>LVASGENKIKQGLLPSLEDLLFYTIAEGQEKIPVHKFITALKSTGLRTSDPRLKECMDMLRLTLQTTSDGVMLDKDLFKKCVQSNIVLLTQAFRRKFVIPDFMSFTSHIDELYESAKKQSGGKVADYIPQLAKFSPDLWGVSVCTVDGQRHSTGDTKVPFCLQSCVKPLKYAIAVNDLGTEYVHRYVGKEPSGLRFNKLFLNEDDKPHNPMVNAGAIVVTSLIKQGVNNAEKFDYVMQFLNKMAGNEYVGFSNATFQSERES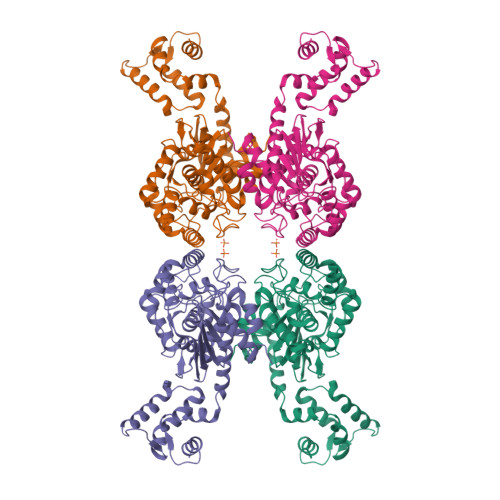GDRNFAIGYYLKEKKCFPEGTDMVGILDFYFQLCSIEVTCESASVMAATLANGGFCPITGERVLSPEAVRNTLSLMHSCGMYDFSGQFAFHVGLPAKSGVAGGILLVVPNVMGMMCWSPPLDKMGNSVKGIHFCHDLVSLCNFHNYDNLRHFAKKLDPRREGGDQRHSFGPLDYESLQQELALKETVWKKVSPESNEDISTTVVYRMESLGEKS[4x]> GPKVEQAVETEPEPELRQQTEWQSGQRWELALGRFWDYLRWVQTLSEQVQEELLSSQVTQELRALMDETMKELKAYKSELEEQLTPVAEETRARLSKELQAAQARLGADMEDVIGRLVQYRGEVQAMLGQSTEELRVRLASHLRKLRKRLLRDADDLQKRLAVYQ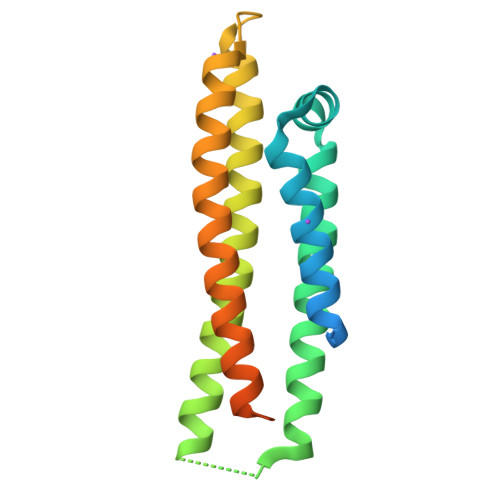AGAREGAERGLSAIRERLGPLVEQGRVR> MSGSMKEEIKRLAEE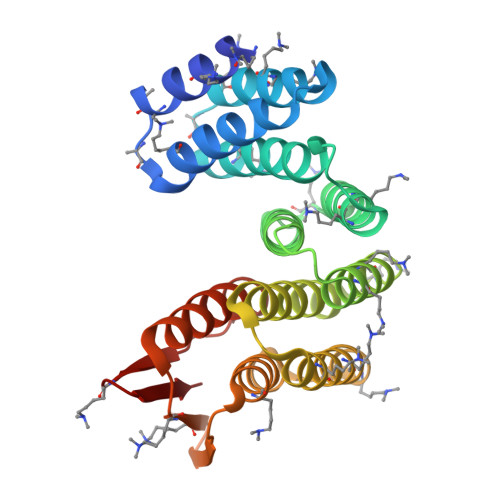LKEKTKNEEIKRLAEEAAELAERSDDPEVLEVVKKALEEALKSKNEEKIELLLLVAVLVAEAGSVDAVEEKLEIALLALKLAEESKDPRIIRGALRAAIAALRSDDPLALKTVKEALERARASKDERLIRAILAAAYAFALLAVAGASAERLKEAEAIVKELIAAAEKGASPQELVLLVIEMMVKGMGVTMETHRSGNEVKVVIKGLHESQQEVLLEAVLFAAELMGVRVRIRFKGDTVTIVV>GPGSTKQVPTEINPKFKDLRAYYTKPSLEFKNEIGIILKKWTTIRFMNVVPDYFIYKIALVGKDDKKYGEGVHRNVDVFVVLEENNYNLEKYSVGGITKSNSKKVDHKAGVRITKEDNKGTISHDVSEFKITKEQISLKELDFKLRKQLIEKNNLYGNVGSGKIVIKMKNGGKYTFELHKKLQENRMAD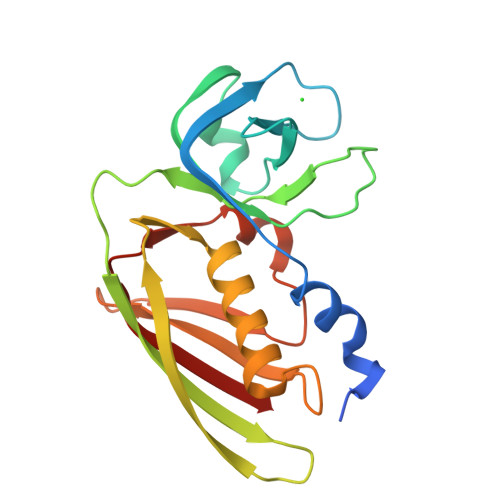VIDGTNIDNIEVNIK[2x]> MSYSAYFAKAGFQFPAGLSALVAGIVALNVCTGRPTKGTKEISNAEYNATPIGYLQSPDQHPTAFPKVPGMKDVHGSPHHHH;> MMRAAQKAKQELPATVLTQTRSYLAPLRSDFTEEITAPKVASASNLVNEWNNKKQATENLMKLLQAYKDIGDAKSEPLLKNHNPRTFEDRDYPVPDFRTQNLKAGDVPKFFDTVISTRASAAIASKDKFWAGRKTEAEAASAKASAAFPRVAVPEWKKGKTVSIENLNTVTDKYAAALVPKRKLALPVLPEGVKKAVEDFAASVGQAKNASEVSELLAKSLAEKAVVTEGGKVVEGFSYVSKAVAAKVIATRRAEVHERLLKLWAKRLLVSPELAIVPLNEFDAQLASKFEGISPKYQELLSAVAQGNKTFAQRLNSSPAFSSFLLKREKAESEVPPSELELEAAQKAAELEDPEVALRTLLGPQMEALGASDLLLSEQIRVITEHRYTPDRLQYKEGMKLADKIAAQEAALKEELKVIYGDNVDVKHFQASPRTPVQQLFDSLKNAAANKERAAKEAAAAASPYLAYAVTKKQEVQADPSNIPFDEVLYPQLSEELLELELSDIREDEIALEKAEEEELWLLTLTQQFKHIQKHFGIDLPHSVVAHMDPLLIKKIDWETTNALEDFDITLDDMGAEDAKEQWGAENLSHHFLPLIRYRRDLARKNGDRYGPDLVNGN;> MRQASRLALSIRQAGNVEAASAVPAMTRQFSAPGSHEHHETPLSKVMPTVVSIPRKVACLALGATKKVVCGLASSGPSQNLVSTFANKVIVEENLVNVAEIDVPFWSYWLSSAGFTSKDAFVKFAEAVKPKVAALSTSDITNLTVAFKRANYYDKDLFTGIEANVSANFTKFETEQLLQIVATFDAFNHSSVAFLDDVADSITYCNHYLAPVRAGADELATLLTYYAKNGHERADLLATVARGFSEVSLGKLSAAQRKDTVLSALKAFQTFGFYPESIEAVIGAALVSPAEYSAEELKEVEAVKVAAENALGGEFVLIQEGAHGH;> MKLLPESLQQEAATAAVVASWVLWHLDTQLLPTIMREHKLHACWAAAAKRYNEKLFKLNPSYDRVLSLPAVSKNQVLENVFHTAPKAPVEHLEKMVSANSKVYDALNLQSKRVLIWQVKPALF;> MMLRTLTRSSAVAGQAVRLFKTSAAAAEGNSVAGIIKSVNETSGANLLSSLKTIKAQAAPIYPAAASSTGYSTQAKIALFGALSWILYRADGQSKAHEWIVDLNLNVLQAAWLISFSSLIPFRAVYFAFRGMAPATASTLNGLKTFSSISL;> MVLGEVYLKDILRTPPTGAIPANVPHPFQTSFYTYATKKLIPRHWYLLGGFTFTITLYGILDGLRDSGK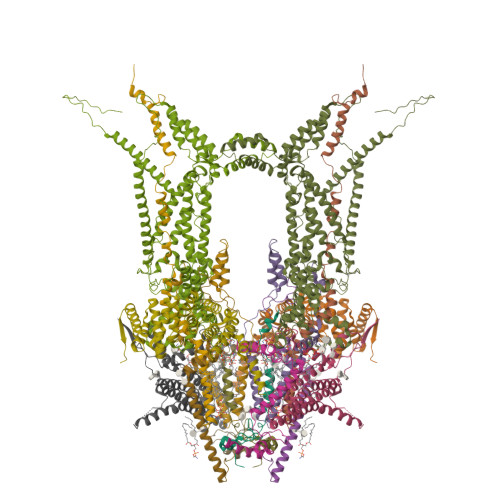KKAYDEAIHAGKTPYTAGGH;> MAVTSFLGKAFEKYFYDFSAYEQFGLNRFLSSKGQYVALRHVGFVMVGVNVLLAANFPFNPPFPTIGMCPAGWEGTWVCQADKAKALEMYKEWKKSN;> MSVLSSVSMGSRIGSSLLGRSSAYLAQCGFSTRSNLNGSIDTSSSVFQALSSDNENKPAASPLNVKLPGMSCSSILLPKTSRIAVPFGNQTMAMSSVRDVKTGSLPTNFLTGVYRFWRSQNPAEKPHDPVNDRLLPAVVDASDKRASIGTWATTFFCTIISCNLLGLMPFNEAPTSGLGFATGLGVSVWATATILGLSKTGFKFPGHFIPGGTPWPMAFIFVPLETISYTFRAVSLGVRLWVNMLAGHTLLHILTGMALALPFSLGFFSMVPATFGVCCLLSALVGLEYLVAVLQSGVFSILSTVYVGEFNHDKFIGPAAKIVKKIH Purine riboside-3',5'-cyclic monophosphate | C10 H11 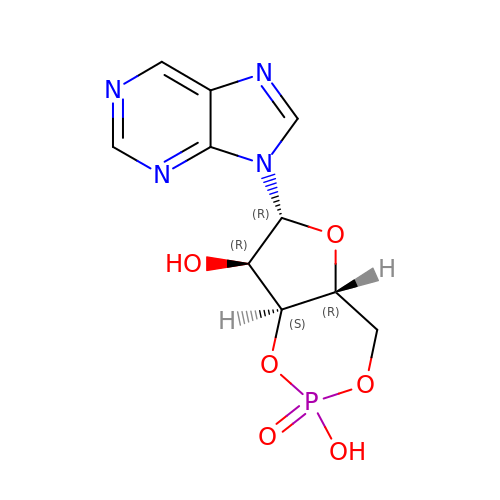N4 O6 P | AVSJXTVPIHQRPY-FDDDBJFASA-N> NSLSVHQLAAQGEMLYLATRIEQENVINHTDEEGFTPLMWAAAHGQIAVVEFLLQNGADPQLLGKGRESALSLACSKGYTDIVKMLLDCGVDVNEYDWNGGTPLLYAVHGNHVKCVKMLLESGADPTIETDSGYNSMDLAV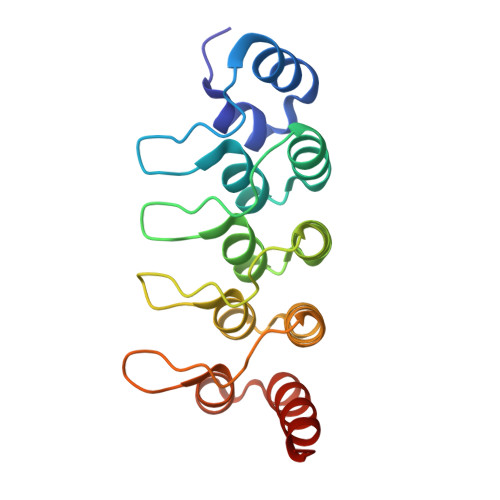ALGYRSVQQVIESHLLKLLQN> HHHHHHENLYFQSMIKQRTLKNIIRATGVGLHSGEKVYLTLKPAPVDTGIVFSRTDLDPVVEIPARAENVGETTMSTTLVKGDVKVDTVEHLLSAMAGLGIDNAYVELSASEVPIMDGSAGPFVFLIQSAGLQEQEAAKKFIRIKREVSVEEGDKRAVFVPFDGFKVSFEIDFDHPVFRGRTQQASVDFSSTSFVKEVSRARTFGFMRDIEYLRSQNLALGGSVENAIVVDENRVLNEDGLRYEDEFVKHKILDAIGDLYLLGNSLIGEFRGFKSGHALNNQLLRTLI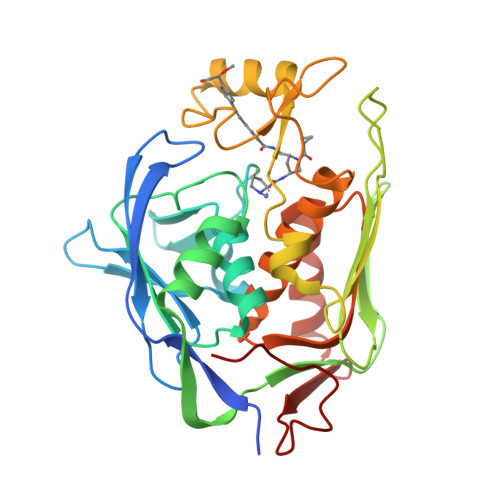ADKDAWEVVTFEDARTAPISYMRP>[2x]GHMENKVINFK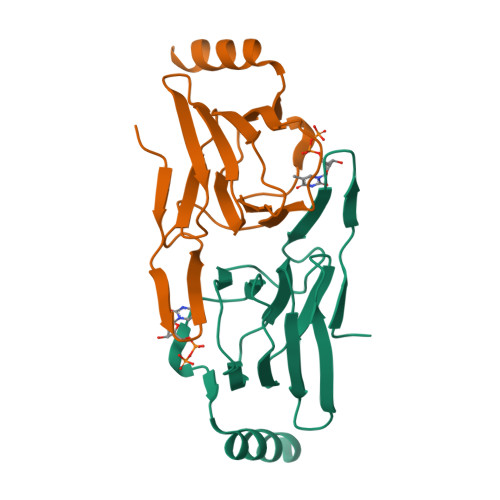KIIDSRGSLVAIEENKNIPFSIKRVYYIFDTKGEEPRGFHANKKLEQVLVCLNGSCRVILDDGNIIQEITLDSPAVGLYVGPAVWHEMHDFSSDCVMMVLASDYYDETDYIRQYDNFKKYIAKINLEKEG N-[(2S)-3-[(R)-(4-bromophenyl)(hydroxy)phosphoryl]-2-{[3-(3'-chlorobiphenyl-4-yl)-1,2-oxazol-5-yl]methyl}propanoyl]-L-alanyl-L-alaninamide 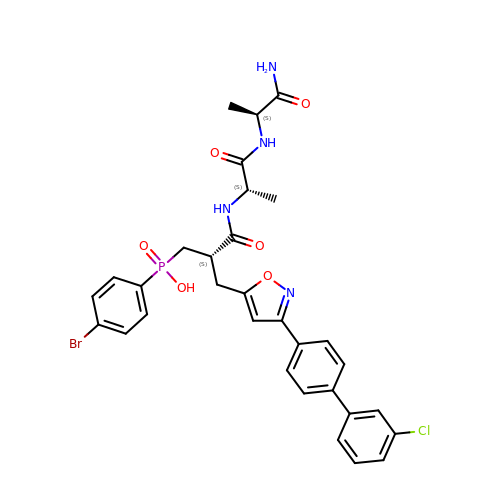| C31 H31 Br Cl N4 O6 P | LIUMDGLYGBIKBM-SFYKDHMMSA-N> MGHHHHHHAQLYACQDPTIFEERHLKYISQLGKGNFGSVELCRYDPLGDNTGALVAVKQLQHSGPD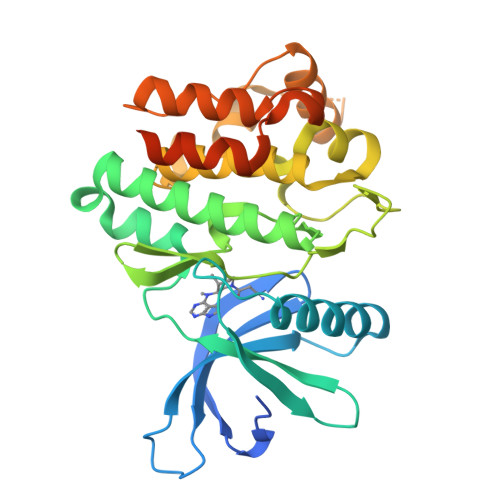QQRDFQREIQILKALHSDFIVKYRGVSYGPGRQSLRLVMEYLPSGCLRDFLQRHRARLDASRLLLYSSQICKGMEYLGSRRCVHRDLAARNILVESEAHVKIADFGLAKLLPLDKDYYVVREPGQSPIFWYAPESLSDNIFSRQSDVWSFGVVLYELFTYCDKSCSPSAEFLRMMGCERDVPALSRLLELLEEGQRLPAPPACPAEVHELMKLCWAPSPQDRPSFSALGPQLDMLWSGSRGCETHAFTAHPEGKHHSLSFS>[2x]MSIIAINENGF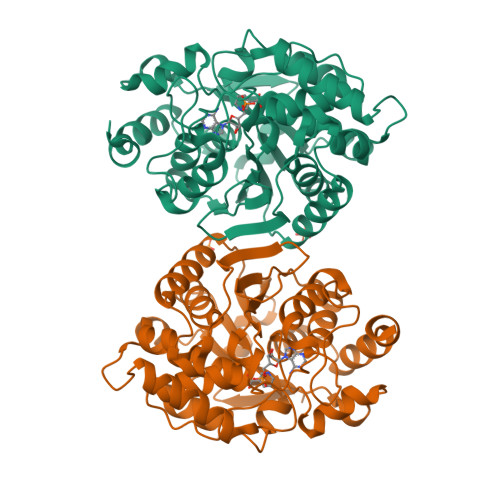LDKIKGRNPLFTCVISSIETTLSIPISGVHRDVIKYTPSADVELVFYGKSLTLKTPPIDATGSPTPATITRACVELKNIKNLHIDAGAFVKPKIPFIEIDEKPTGRIEEGKAMNNSKELYMKGYLLGKNLDAELLIVGESVPGGTTTALGVLLGLGYDAEGKVSSGSINNPHELKIKVVREGLKKAGINEKSSVFDVLNAVGDKMMPVVAGLAISFAERNKPVILAGGTQMSAVLAVIKEINKKVLDKNLIAIGTTEFVLNDKKGDLKGIVEQIGNVPVLASKFYFEKAKIEGLKNYCKGSVKEGVGAGGIAVYSIVNDLEPTKIREFIENKFYEWYKE4-(7-methoxyquinolin-4-yl)-2-methyl-phenol | C17 H15 N O2 | 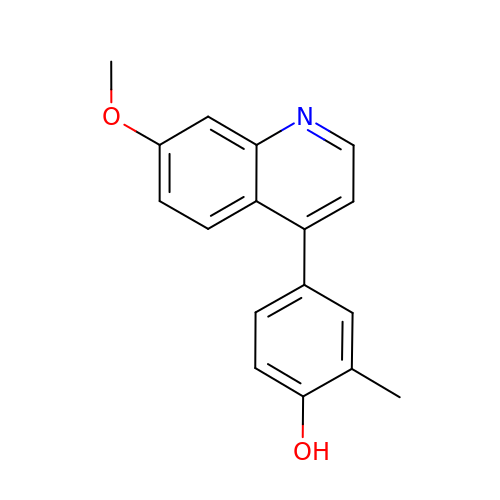HNYBTVKYLVLWCB-UHFFFAOYSA-N> GSERRAVYIGALFPMSGGWPGGQACQPAVEMALEDVNSRRDILPDYELKLIHHDSKCDPGQATKYLYELLYNDPIKIILMPGCSSVSTLVAEAARMWNLIVLSYGSSSPALSNRQRFPTFFRTHPSATLHNPTRVKLFEKWGWKKIATIQQTTEVFTSTLDDLEERVKEAGIEITFRQSFFSDPAVPVKNLKRQDARIIVGLFYETEARKVFCEVYKERLFGKKYVWFLIGWYADNWFKIYDPSINCTVDEMTEAVEGHITTEIVMLNPANTRSISNMTSQEFVEKLTKRLKRHPEETGGFQEAPLAYDAIWALALALNKTSGGGGRSGVRLEDFNYNNQTITDQIYRAMNSSSFEGVSGHVVFDASGSRMAWTLIEQLQGGSYKKIGYYDSTKDDLSWSKTDKWIGGSPPADQTLVIKTFRFLSQKLFISVSVLSSLGIVLAVVCLSFNIYNSHVRYIQNSQPNLNNLTAVGCSLALAAVFPLGLDGYHIGRNQFPFVCQARLWLLGLGFSLGYGSMFTKIWWVHTVFTKKEEKKEWRKTLEPWKLYATVGLLVGMDVLTLAIWQIVDPLHRTIETFAKEEPKEDIDVSILPQLEHCSSRKMNTWLGIFYGYKGLLLLLGIFLAYETKSVSTEKINDHRAVGMAIYNVAVLCLITAPVTMILSSQQDAAFAFASLAIVFSSYITLVVLFVPKMRRLITRGEWQSEAQDTMKTGSSTNNNEEEKSRLLEKENRELEKIIAEKEE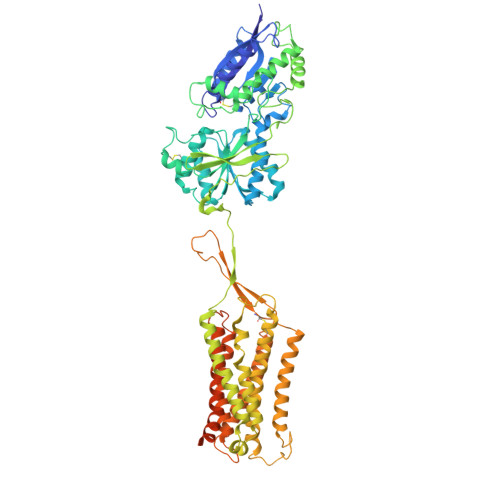RVSELRHQLQSRLEVLFQ N-[3,4-bis(fluoranyl)phenyl]methanesulfonamide | C7 H7 F2 N O2 S | 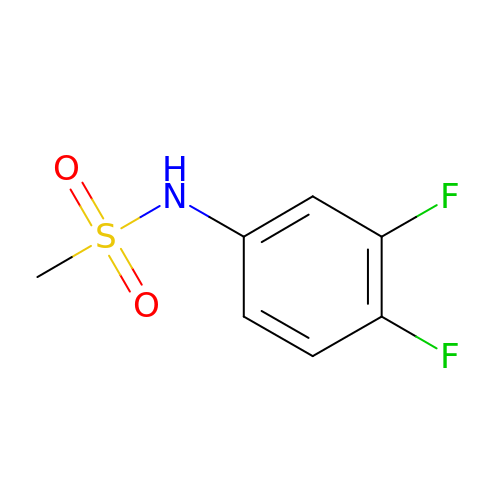CRLGPRNTBCRIBM-UHFFFAOYSA-N>[2x]MELENIVANSLLLKARQGGYGKKSGRSKKWKEILTLPPVSQCSELRHSIEKDYSSLCDKQPIGRRLFRQFCDTKPTLKRH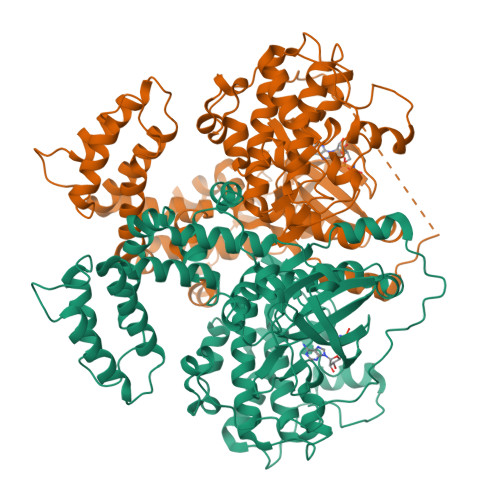IEFLDAVAEYEVADDEDRSDCGLSILDRFFNDKLAAPLPEIPPDVVTECRLGLKEENPSKKAFEECTRVAHNYLRGEPFEEYQESSYFSQFLQWKWLERQPVTKNTFRHYRVLGKGGFGEVCACQVRATGKMYACKKLQKKRIKKRKGEAMALNEKRILEKVQSRFVVSLAYAYETKDALCLVLTIMNGGDLKFHIYNLGNPGFDEQRAVFYAAELCCGLEDLQRERIVYRDLKPENILLDDRGHIRISDLGLATEIPEGQRVRGRVGTVGYMAPEVVNNEKYTFSPDWWGLGCLIYEMIQGHSPFKKYKEKVKWEEVDQRIKNDTEEYSEKFSEDAKSICRMLLTKNPSKRLGCRGEGAAGVKQHPVFKDINFRRLEANMLEPPFCPDPHAVYCKDVLDIEQFSVVKGIYLDTADEDFYARFATGCVSIPWQNEMIESGCFKDINKSESEEALPLDLDKNIHTPVSRPNRGFFYRLFRRGGSLTMVPSEKEVEPKQSENLYFQ> MAFEENLYCDYTPGAAKAVAGKDVILAVFNAAGDKLLAVAGQQGLTVNRSKDSIEITSKDTVGGWKSKIGGMKEWSIENDGLYVADAESHKELAKYFESDSPVCVKIINQASKKGLFGGLAIVADYSFEAPFDEAMTYSVKLDGM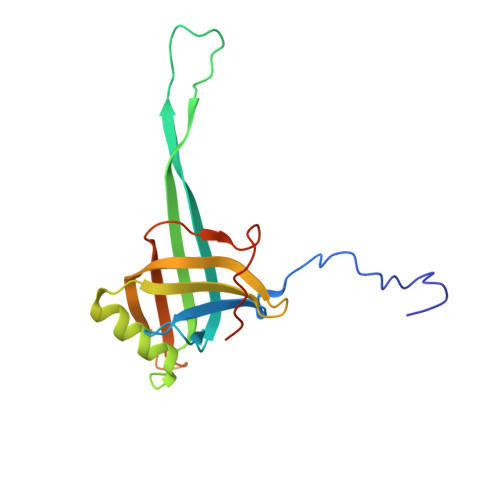GALVDLTITEGGDQMPGETPVAPAE> MEGVLYKWTNYLTGWQPRWFVLDNGILSYYDSQDDVCKGSKGSIKMAVCEIKVHSA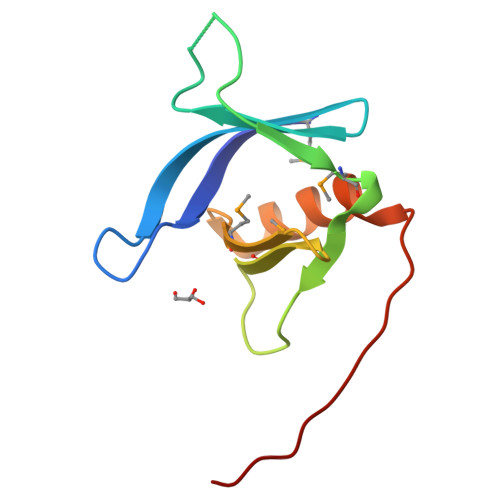DNTRMELIIPGEQHFYMKAVNAAERQRWLVALGSSKASLTDTRLVPR>MVKREFPPGFWKDDLIDSLTSSHKVAASDEKRIETLISEIKNMFRCMGYGETNPSAYDTAWVARIPAVDGSDNPHFPETVEWILQNQLKDGSWGEGFYFLAYDRILATLACIITLTLWRTGETQVQKGIEFFRTQAGKMEDEADSHRPSGFEIVFPAMLKEAKILGLDLPYDLPFLKQIIEKREAKLKRIPTDVLYALPTTLLYSLEGLQEIVDWQKIMKLQSKDGSFLSSPASTAAVFMRTGNKKCLDFLNFVLKKFGNHVPCHYPLDLFERLWAVDTVERLGIDRHFKEEIKEALDYVYSHWDERGIGWARENPVPDIDDTAMGLRILRLHGYNVSSDVLKTFRDENGEFFCFLGQTQRGVTDMLNVNRCSHVSFPGETIMEEAKLCTERYLRNALENVDAFDKWAFKKNIRGEVEYALKYPWHKSMPRLEARSYIENYGPDDVWLGKTVYMMPYISNEKYLELAKLDFNKVQSIHQTELQDLRRWWKSSGFTDLNFTRERVTEIYFSPASFIFEPEFSKCREVYTKTSNFTVILDDLYDAHGSLDDLKLFTESVKRWDLSLVDQMPQQMKICFVGFYNTFNDIAKEGRERQGRDVLGYIQNVWKVQLEAYTKEAEWSEAKYVPSFNEYIENASVSIALGTVVLISALFTGEVLTDEVLSKIDRESRFLQLMGLTGRLVNDTKTYQAERGQGEVASAIQCYMKDHPKISEEEALQHVYSVMENALEELNREFVN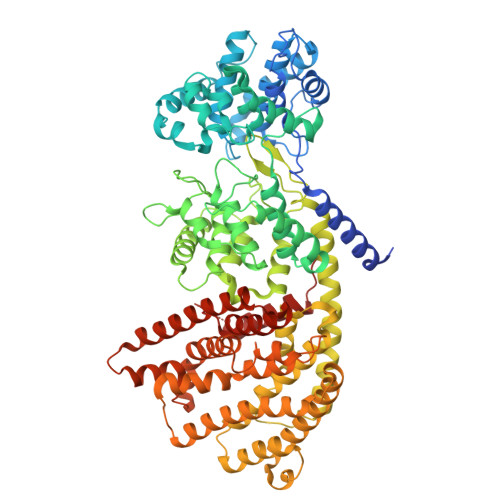NKIPDIYKRLVFETARIMQLFYMQGDGLTLSHDMEIKEHVKNCLFQPVA[4x]Here, we determine mycobacterial MsRv1273c/72c to be an isoniazid efflux pump and determine several structures by cryo-electron microscopy showing specific asymmetrical features including an N-terminal extending loop and a periplasmic helical hairpin only found in MsRv1272c. Thus, MsRv1273c should have a degenerate site impaired for ATPase activity while MsRv1272c has a functional consensus site with the classic enzymatic motifs. Confirmation that this is correct was achieved by mutating both E553Q and D497N, creating the double mutant, which has little activity. Together, these results indicate that the consensus site of MsRv1273c/72c is functional with normal ATPase activity while its degenerate site exhibits very low activity. Thus, MsRv1273c/72c is a drug efflux pump for isoniazid, but not ethambutol.

An approach to obtain the Occ state of ABC transporter is to inactivate the ATPase activity by making a glutamate to glutamine (EtoQ) mutation in the Walker B motif of NBD. Based on this, we purified the E553Q mutant which had a significantly diminished ATPase activity and then added ATP before data collection. We then solved the cryo-EM structure of E553Q mutant in the presence of ATP at 3.1 Å resolution, which showed an ATP-bound Occ state. In the Occ structure, the central cavity in the TM region is sealed at both the cytoplasmic and periplasmic sides. The N-terminal extending loop is squeezed out from the cavity. The two NBDs are fully closed and interact with each other in an antiparallel manner. ATP is clamped between the dimer interface at the consensus and degenerate NBSs. The binding mode of ATP is similar at both sites and is classical amongst the ABC transporter family. Taking ATP binding at the degenerate site for example, the α- and β-phosphate group of ATP binds in the groove formed by Walker A motif of MsRv1273c, while the γ-phosphate group is stabilized by Mg2+ and helix α6 of MsRv1272c. In the ATP-bound Occ structure, the NBDs are fully dimerized with distances of 6.8 Å and 6.1 Å at the two NBSs.

> SNMLWALLRQYVRPYRWLLAVVAVLQVISNMASLYLPTVNAAIIDDGVAKGDTARIVELGAVMLGVTALQVVCAVGAVFFGARAATGFGHDLRAAVFTHVTTFSAEEAGRFGAASLLTRTTNDVGHIQQLVQLTVTMLITAPIMSIGGIFMALHQDAGLSWLLLVSVPVLGLANYWIIRHLMPVFTRMQSLIDGINRVLRDQLSGIRVIRAFAREPLERVRFAEANQTLSDSALEAGRWQALMLPVTTLVINVSSVALIWFGGLRIDAGQMQVGSLIAFLAYFMQILMAVLMATFMLVIFPRAAVCADRIGEVLSTQTAITNPADPVRPAAIAGDIGVHDATFCYPGADRPVLQDVSFTVPRGTTTAVVGSTGSGKSTLISLICRLYDVTSGSLRIDGVDVRDLDIEQLWSAIGLVPQRGYLFSGTVAENLRYGRADATDDEMWEALRVAAAADFVRAHPQGLDMPVAQGGINFSGGQRQRLAIARAVIRRPAIYLFDDAFSALDVHTDARVRDALREVAADATVVIVSQRISTVIEADQVVVIDDGRVVGIGTHDTLLADCPIYAEFAESQAL;> TRDFKGSAIRLARRLLPQRALTLAVILLGVGGIAIGVIGPRILGHATDLLFNGVIGRELPAGLTKEQAVEAARARGDGTFADLLSGMDIVPGQGVDFGAVGRTLALALGLYLVAALLVWVQARLLNVTVQRTMVALRAEVQEKIHRLPLSYFDSRQRGEVLSRVTNDVDNIQNSVSMTISQLLTSVLTVFAVLVMMLTISPLLTLFTVVTVPASLWVTRWITRRSQPLFVAQWRNTGRLAAHLEETYSGFTIVKTFGHREAAAGKFAELNSETQQSSFGAQFFSGLVSPATMFIGNLSYVAVAVVGGLQVATGQITLGSIQAFIQYVRQFNQPLTQVAGMYNTLQSGIASAERVFDLLDTEEESADSPRRADVRTGRVEFEHVSFSYVPGTPVIEDLSLVAEPGSTVAIVGPTGAGKTTLVNLLMRFYDVDSGRITIDGVDIASVSRESLRASIGMVLQDTWLFAGTIYDNIAYGRPDADEDEVIEAATAAYVDRFVHTLPNGYDTRVDDDGGAISAGEKQLITIARAVLARPKLLVLDQATSSVDTRTELLIAHAMAELRRDRTSFIIAHRLSTIRDADLILVMDSGRIIERGTHEELLARHGRYWEMTRVHLGG>[2x]PQGPEIRRAADNLEAAIKGKPLTDVWFAFPQLKTYQSQLIGQHVTHVETRGKALLTHFSNDLTLYSHNQLYGVWRVVDTGEEPQTTRVLRVKLQTADKTILLYSASDIEMLRPEQLTTHPFLQRVGPDVLDPNLTPEVVKERLLSPRFRNRQFAGLLLDQAFLAGLGNYLRVEILWQVGLTGNHKAKDLNAAQLDALAHALLEIPRFSYATRGQVDE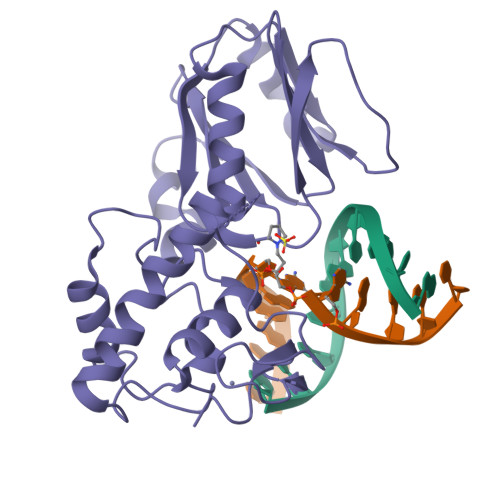NKHHGALFRFKVFHRDGEPCERCGSIIEKTTLSSRPFYWCPGCQH>[2x]SNAQEKVGTIGIAIPSATHGFMGGLNFHAQDTIKRLQEVYPQLDFVLATAGNAGKMVNDIE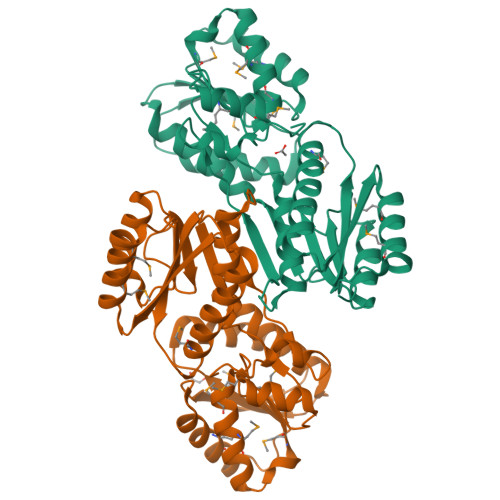DMVATRNISALVVLPFESEPLTSPVQAVKEAGIWVTVVDRGLSVEGIEDLYVAGDNPGFGRVAGEYFAQHLESGKKIVVLRGIPTTLDNERVEAFTAAIEGSGIEVLDMQHGNWNRDDAFNVMQDFLSKYPQIDAVWAADDDMAIGAMEAIAQAGRTEEMWVMGGAGMKEIIRRIADGDPQLPANVTYPPAQISTAIELTALKLVSSTPVSGRFIIGSQLVTPENAEQFYFPDSPF> DQLICVNENGGCEQY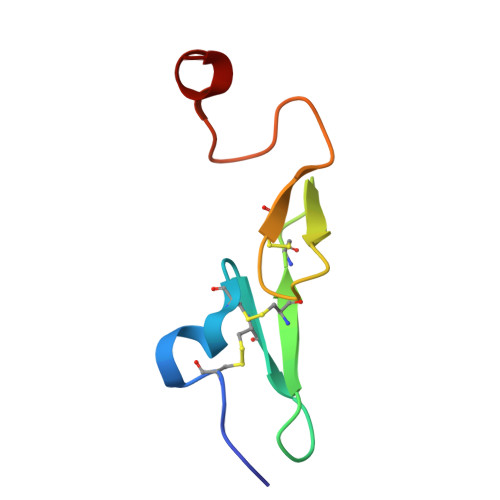CSDHTGTKRSCRCHEGYSLLADGVSCTPTVEYPCGKIPILEKR>[6x]GHMNDLI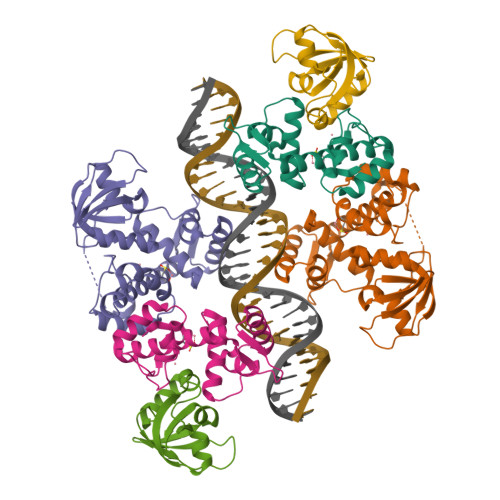DTTEMYLRTIYDLEEEGVVPLRARIAERLEQSGPTVSQTVARMERDGLLTVAEDRHLELTKAGRARAISVMRKHRLAERLLVDVIGLEWEQVHLEACRWEHVMSEAVERKLVKLLGNPTTSPYGNPIPGLDELGVGDSVEPVDTDLRRVDEVARSGGGRALVCRIAEHVQLDPDLMSELKKVGVVPGNEIDIVAVAGVNKPIQVQGSEGGTQLQPGIAHAVMVRVK> MGHHHHHHMSADFGLIGLAVMGQNLILNAADHGFTVCAYNRTQSKVDHFLANEAKGKSIIGATSIEDFISKLKRPRKVMLLVKAGAPVDALINQIVPLLEKGDIIIDGGNSHFPDSNRRYEELKKKGILFVGSGVSGGEEGARYGPSLMPGGSEEAWPHIKNIFQSISAKSDGEPCCEWVGPAGAGHYVKMVHNGIEYGDMQLICEAYDIMKRLGGFTDKEISDVFAKWNNGVLDSFLVEITRDILKFDDVDGKPLVEKIMDTAGQKGTGKWTAINALDLGMPVTLIGEAVFARCLSALKNERIRASKVLPGPEVPKDAVKDREQFVDDLEQALYASKIISYAQGFMLIREAAATYGWKLNNPAIALMWRGGCIIRSVFLGQITKAYREEPDLENLLFNKFFADAVTKAQSGWRKSIALATTYGIPTPAFSTALSFYDGYRSERLPANLLQAQRDYFGAHTFRVLPECASDNLPVDKDIHINWTGHGGNVSSSTYQA

The 6-phosphogluconate dehydrogenase (6PGDH, EC 1.1.1.44) is the third enzyme of the oxidative branch of the pentose phosphate pathway. The 6PGDH catalyzes the oxidative decarboxylation of 6-phosphogluconate (6PG) to ribulose 5-phosphate (Ru5P) and CO2 with the concomitant reduction of NADP+ to NADPH. Prokaryotic and eukaryotic 6PGDHs are generally homodimers, with a monomer of ~470 amino acids and a molecular weight of ~52 kDa. Each subunit is comprised of an N-terminal Rossmann fold coenzyme-binding domain, a large all-helical domain and a small C-terminal tail.

Moreover, we determined the crystal structure of Gnd1 in complex with two citrate molecules by molecular replacement and refined it to 2.37 Å resolution. Similar to the 6PGDHs reported in other species, Gnd1 forms dimer. The dimer is formed by the C-terminal tail of two subunits threading through each other forming a mobile lid on the substrate binding pocket. To our surprise, two citrate molecules were bound to the active site of each Gnd1 monomer. The negative charges between two citrate molecules lead to electrostatic repulsion, so they occupy a larger space than 6PG. Previous study has shown that citrate serves as an inhibitor of 6PGDH. Our current research provides for the first time the conformation of 6PGDH bound with an inhibitor. From the structure of Gnd1 we found two highly conserved residues, Arg446 and His452, to be vitally important for citrate binding. These two residues were also shown to be critical for 6PG binding from structural studies of sheep liver 6PGDH. We further studied the role of the Gnd1 C-terminal tail and found that it is dispensable for dimerization, but crucial for the enzymatic activity.>HAALRQPQVAELLAEARRAFREEFGAEPELAVSAPGRVNLIGEHTDYNQGLVLPMALELMTVLVGSPRKDGLVSLLTTSEGADEPQRLQFPLPTAQRSLEPGTPRWANYVKGVIQYYPAAPLPGFSAVVVSSVPLGGGLSSSASLEVATYTFLQQLCPDSGTIAARAQVCQQAEHSFAGMPCGIMDQFISLMGQKGHALLIDCRSLETSLVPLSDPKLAVLITNSNVRHSLASSEYPVRRRQCEEVARALGKESLREVQLEELEAARDLVSKEGFRRARHVVGEIRRTAQAAAALRRGDYRAFGRLMVESHRSLRDDYEVSCPE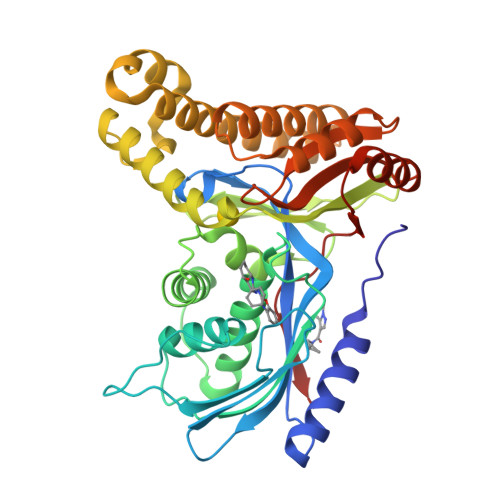LDQLVEAALAVPGVYGSRMTGGGFGGCTVTLLEASAAPHAMRHIQEHYGGTATFYLSQAADGAKVLCL[4x]> GSHMADPGDRLGVLTTTRRVVEQAQAVWIDHDAVAQIAEAFAARQVTPPTWNRELHWSDGREALANYILVLDAVNFCFWGEPRWRIEYAGAVYDGYWALAAS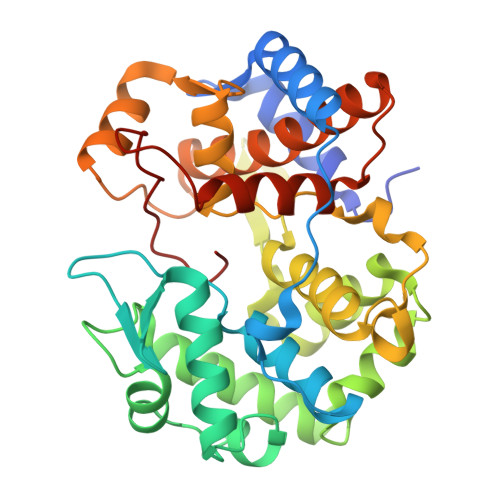LKRALEQGVPLTDASYLAEITRDDVATIFAGEGEIPLLDERARILRETGSVLAERFAGRFSDAIAAAGRSAVALVDIVTNAFPSFRDVATYRGEQVRFYKRAQILVSDLYGAFDGSDLGAFDDLGELTAFADYKVPQVLHHLGILRYAPALHDRLARREEIPAGSPEEVEIRAATIWGVEELRRALASRGHALDAYQVDWLLWDEGQRLPAGTLPYHRTRTIFY> MLGILNKMFDPTKRTLNRYEKIANDIDAIRGDYENLSDDALKHKTIEFKERLEKGATTDDLLVEAFAVVREASRRVTGMFPFKVQLMGGVALHDGNIAEMKTGEGKTLTSTLPVYLNALTGKGVHVVTVNEYLASRDAEQMGKIFEFLGLTVGLNLNSMSKDEKREAYAADITYSTNNELGFDYLRDNMVLYKEQMVQRPLHFAVIDQVDSILIDEARTPLIISGQAAKSTKLYVQANAFVRTLKAEKDYTYDIKTKAVQLTEEGMTKAEKAFGIDNLFDVKHVALNHHINQALKAHVAMQKDVDYVVEDGQVVIVDSFTGRLMKGRRYSEGLHQAIEAKEGLEIQNESMTLATITFQNYFRMYEKLAGMTGTAKTEEEEFRNIYNMQVVTIPTNRPVVRDDRPDLIYRTMEGKFKAVAEDVAQRYMTGQPVLVGTVAVETSELISKLLKNKGIPHQVLNAKNHEREAQIIEEAGQKGAVTIATNMAGRGTDIKLGEGVKELGGLAVVGTERHESRRIDNQLRGRSGRQGDPGITQFYLSMEDELMRRFGAERTMAMLDRFGMDDSTPIQSKMVSRAVESSQKRVEGNNFDSRKQLLQYDDVLRQQREVIYKQRFEVIDSENLREIVENMIKSSLERAIAAYTPREELPEEWKLDGLVDLINTTYLDEGALEKSDIFGKEPDEMLELIMDRIITKYNEKEEQFGKEQMREFEKVIVLRAVDSKW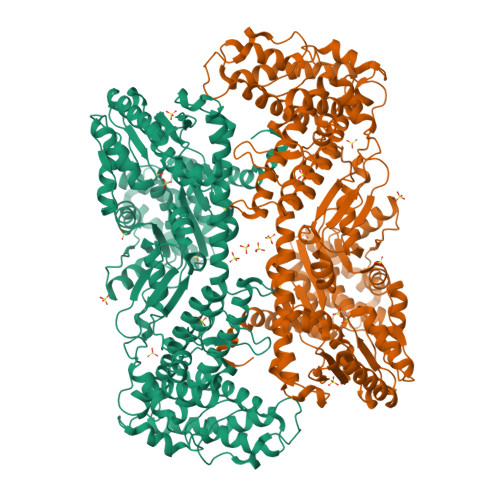MDHIDAMDQLRQGIHLRAYAQTNPLREYQMEGFAMFEHMIESIEDEVAKFVMKAEIENNLEREEVVQGQTTAHQPQEG>[4x]MAHHHHHHMVNVAVIGAAGGIGQSLSLLLLRELPFGSTLSLYDVVGAPGVAADLSHIDRAGITVKHAAGKLPPVPRDPALTELAEGVDVFVIVAGVPRKPGMTRDDLFNVNAGIVMDLVLTCASVSPNACFCIVTNPVNSTTPIAAQTLRKIGVYNKNKLLGVSLLDGLRATRFINNARHPLVVPYVPVVGGHSDVTIVPLYSQIPGPLPDESTLKEIRKRVQVAGTEVVKAKAGRGSATLSMAEAGARFTMHVVKALMGLDTPMVYAYVDTDGEHECPFLAMPVVLGKNGIERRLPIGPITTVEKEMLEEAVGVVKKNIAKGETFARSKL;> MAHHHHHHMDCSTGAAIGQQFAKDAFHMHGGVGVGPTGNSEHDVLMNEMMMVQTPTGPAGEWTHQFAAYQGQQQQQQQQHPQELAMRHQQNDAFMLRQQQEMEEAFCTFCTTHPHSHAHSHQPQGLVGPAMMGPQIMPPMMFGPGTGGFMMGAPPMMPYASMKFAGDAAMAAANNTNMTQGATATSTTSVQQELQQQSSDNGWVEKLRDAEWAQDYSDAQVFTLEGQSEQTMEEHAKNSEFYQFMDKIRSKELLIDEETGQLVQGPGPDPDAPEDAEYLKEWAAAEGLNMPPGFFEHMMQRPQGNNEQAEGRLFDGSNDALMDDGALDNAADVEEWVREYAEAQEQLQRVQNETNYPFEPNNPYMYHDKPMEEGIAMLQLANMAEAALAFEAVCQKEPENVEAWRRLGTTQAENEKDCLAIIALNHARMLDPKDIAVHAALAVSHTNEHNVGAALQSLRSWLLSQPQYEHLGLVDLREVAADEGLDEVPEENYFFAAPSEYRDCCTLLYAAVEMNPNDPQLHASLGVLHNLSHRFDEAAKNFRRAVELRPDDAHMWNKLGATLANGNRPQEALEAYNRALDINPGYVRVMYNMAVSYSNMAQYPLAAKHITRAIALQAGGTNPQGEGSRIATRGLWDLLRMTLNLMDRSDLVEASWQQDLTPFLREFGLEEMAV

Having no protein synthetic abilities, peroxisomes import all required enzymes from the cytosol through a peroxin (Pex) import system. Peroxisome targeting sequence 1 (PTS1)-tagged cargo is recognized by cytosolic receptor, Pex5. The cargo-Pex5 complex docks at the peroxisomal membrane translocon, composed of Pex14 and Pex13, facilitating translocation into the peroxisomal lumen. MDH is a crucial enzyme for the glycolysis auxiliary pathway, maintaining the pool of malate/oxaloacetate.

We successfully reconstructed MP1 and MP2 maps showing one and two copies of Pex5 bound to MDH tetramer, respectively. MP1 and MP2 maps show a well-resolved MDH region, but poorly resolved Pex5 region(s), indicating conformational heterogeneity in the latter component. The refined maps facilitated model building of MDH and Pex5 residues 327–462 and 487–653, encompassing the TPR domain and an upstream helix containing the Wxxx(F/Y) motif (residues 327–345). The helix distinguishes our structure from previously available Pex5 TPR domain crystal structures, in which the Wxxx(F/Y) motif-containing helix is not resolved. Recognition of the MDH by Pex5 is mediated via PTS1 motif at the central cavity of Pex5 TPR domain. Along PTS1-mediated interaction, two additional interfaces between MDH and Pex5 TPR domain are identified by PISA analysis. Interface 1 involves MDH residues 62–70 and Pex5 residues 439–444, forming a loop connecting α6 and α7. To clarify the ambiguity, we reconstituted in vitro and solved the structure of the MDH-Pex5 binary complex devoid of Pex14NTD. The map for the binary complex revealed no density beyond the MDH and Pex5 TPR domain, indicating that the additional density observed in the ternary complex originates from Pex14NTD.~{N}-[[[2-methyl-4-(3-methylbutyl)phenyl]amino]methyl]hydroxylamine | C13 H22 N2 O | 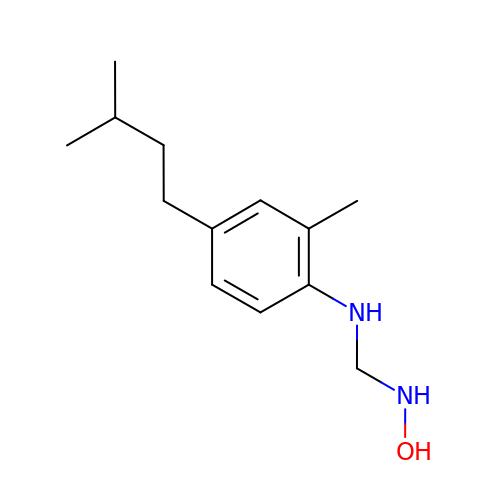BNHIDDHQCYEQMT-UHFFFAOYSA-N> GMVRRTRAEMEETRATLLATARKVFSERGYADTSMDDLTAQASLTRGALYHHFGDKKGLLAAVVEQIDAEMDERLQAISDTAEDDWEGFRCRCRAYLEMALEPEIQRIVLRDARAVLGGASPDSQRHCVESMQRLIDNLIRQGVVAEADPQALASLIYGSLAEAAFWIAEGEDGNARLAQGVAALELLLRGLLV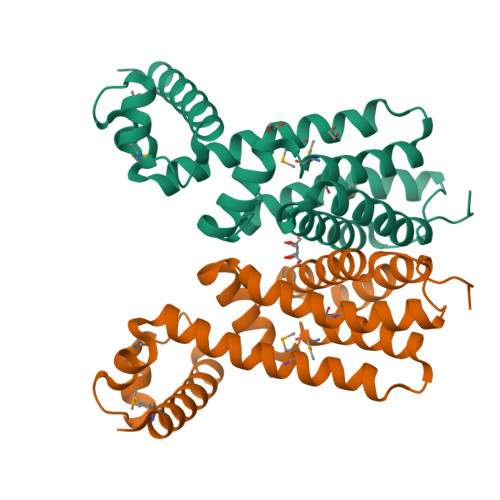KPR>MELRHLRYFVAVVEEQSFTKAADKLCIAQPPLSRQIQNLEEELGIQLLERGSRPVKTTPEGHFFYQYAIKLLSNVDQMVSMTKRIASVEKTIRIGFVGSLLFGLLPRIIHLYRQAHPNLRIELYEMGTKAQTEALKEGRIDAGFGRLKISDPAIKHTLLRNERLMVAVHASHPLNQMKDKGVHLNDLIDEKILLYPSSPKPNFSTHVMNIFSDHGLEPTKINEVREVQLALGLVAAGEGISLV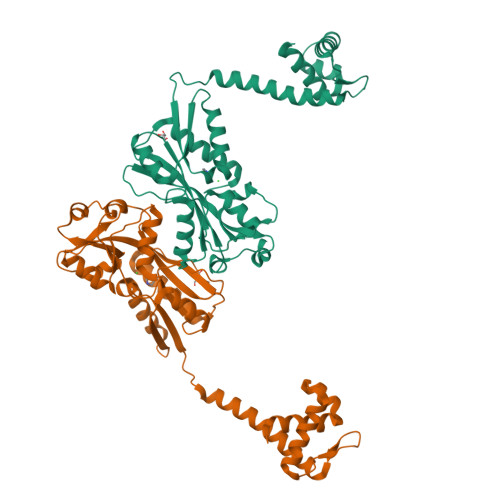PASTQSIQLFNLSYVPLLDPDAITPIYIAVRNMEESTYIYSLYETIRQIYAYEGFTEPPNWLEHHHHHH[2x]> KGSVVIVGRINLSGDTAYAQQTRGAAACQETSQTGRDKNQVEGEVQIV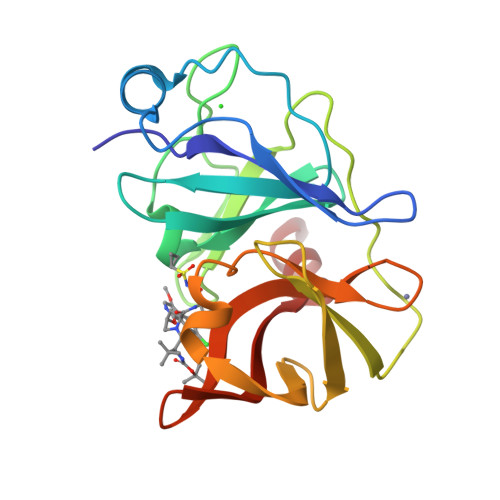STATQTFLATSINGVLWTVYHGAGTRTIASPKGPVTQMYTNVDKDLVGWQAPQGSRSLTPCTCGSSDLYLVTRHADVIPVRRRGDSRGSLLSPRPISYLKGSSGGPLLCPAGHAVGIFRAAVSTRGVAKAVDFIPVESLETTMR> MRSDGRKEDQLRPVSIQRDFLEYPEGSCLI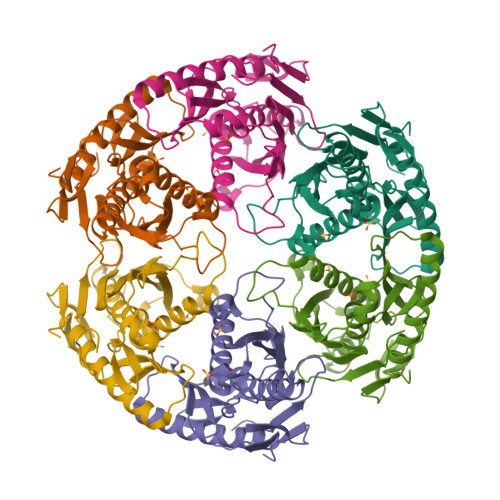SFGKTKVICTASVIENVPNWLKGKGQGWITAEYSMLPRATQQRTIRESVQGRIGGRTHEIQRMIGRAMRTAVELTKIGERTIWVDCDVIQADGGTATAAITGAFVAVADAIIKLHKEGIIEETPIKDFVAAVSVGIVNDRILLDLNFEEDSAAQVDMNVVGTGSGRLSEVHTMGEEYSFTKDELIKMLDLAQKGINELIELQKKLYVIQDGKWERSELKEVSSTT Iripin-4, one of the many salivary serpins from Ixodes ricinus ticks with an as-yet unexplained function, crystallized in two different structural conformations, namely the native partially relaxed state and the cleaved serpin. To inhibit the target protease, serpins undergo a fundamental conformational change that leads to inactivation of both the protease and the serpin itself. The amino acids in the RCL, particularly the residues at the P1 and P1′ positions, determine the protease selectivity of serpins by mimicking the substrate of the target protease. However, Iripin-4 was shown to inhibit only granzyme B protease, as no other protease tested was confirmed to be inhibited.

The structure of native Iripin-4 was solved at 2.3 Å resolution and the crystal belonged to space group P3121 (No. 152), with unit-cell parameters a = 77.78, b = 77.78, c = 109.49 Å, α = 90.0, β = 90.0, γ = 120.0°. The crystal contained one molecule in the asymmetric unit with 51.33% solvent content and a Matthews coefficient of 2.53 Å3 Da−1. The crystal structure has a tentatively assigned nickel cation (Ni2+) located between two molecules of Iripin-4 with crystallographic symmetry that interacts with His253 and Asp257 of both molecules.

> LHEDRLTLANNRFAISLLHNLPTSTETNIFFSPYSISVALGMAFAGARGETREDLFQGFGYPRSDIDDDAVLEAYASQTRRLKSLRSNSTLDAAIGAAIHERISLLSSFEDVLNNSFGADILKVDFINGGQAAVDVINGWVHRKTRGKINLLFGEPLETIIRLVLLNAIYFKGTWDTVFDQRLTTKKPFMNACSTPTEVDTMRGEVYVRHKSFPLLGVDIAEIPYRGMDYSMTILLPTRIDGAEVLKRNITEHLLQDLVKQLVEQQVTVYLPKFKLETEYLLKDHLKKLGINRIFGSGADFSGITHDANLAVSDVVHKTVLEVHEAGTEAAGATGVIIVAESLVESVEFRVDHPFIFFIRNTQTKDILFVGQVNHL>MPACCSWNDVLQYETNKVTRIQSTNYGTVKWVLHMIVFSYISFALVSDKLYQRKEPVISSVHTKVKGIAEVTENVTEGGVTKLGHSIFDTADYTFPLQGNSFFVMTNYVKSEGQVQTLCPEYPRRGAQCSSDRRCKKGWMDPQSKGIQTGRCVPYDKTRKTCEVSAWCPTEEEKEAPRPALLRSAENFTVLIKNNIHFPGHNYTTRNILPTMNGSCTFHKTWDPQCSIFRLGDIFQEAGENFTEVAVQGGIMGIEIYWDCNLDSWSHHCRPRYSFRRLDDKNTDESFVPGYNFRYAKYYKENNVEKRTLIKAFGIRFDILVFGTGGKFDIIQLVVYIGSTLSYFGLATVCIDLLINTYSSAFCRSGVYPYCKCCEPCTVNEYYYRKKCESIMEPKPTLKYVSFVDEPHIRMVDQQLLGKSLQVVKGQEVPRPQMDFSDLSRLSLSLHDSPLTPGQSEEIQLLHEEVAPKSGDSPSWCQCGNCLPSRLPEQRRALEELCCRRKPGRCITTSKLFHKLVLSRDTLQLLLLYQDPLLVLGEEATNSRLRHRAYRCYATWRFGSQDMADFAILPSCCRWRIRKEFPKTEGQYSGFKYPY[3x]

The P2X7 receptor is an ATP-gated ion channel that activates inflammatory pathways involved in diseases such as cancer, atherosclerosis, and neurodegeneration. When present in high concentrations, such as in pathological inflammatory states, extracellular ATP acts as a danger signal to cells by binding to and activating the P2X7 receptor (P2X7R). This spatiotemporal signaling stimulates the innate immune system by triggering assembly of the NLRP3 inflammasome and subsequent cytokine release, as well as activation of various less understood signaling cascades, ultimately resulting in apoptosis. P2X7R antagonists bind to either classical or extended allosteric ligand-binding sites that exist within the extracellular domain at the interface of two protomers.

To characterize the molecular differences between key mammalian P2X7R orthologs, we obtained cryo-EM structures of the full-length wild-type mP2X7 (2.5 Å) and hP2X7 (2.5 Å) receptors in the apo closed state conformation. Conserved features include their trimeric architecture, the 310-helices forming a closed gate, a partially hydrated sodium ion present in the closed pore, palmitoylation of residues in the C-cys anchor, and zinc and guanosine nucleotide-binding sites in the cytoplasmic ballast. There are also hydrogen bonds between the hemisuccinate group of the outer CHS molecule and the side chains of N261, H268, and K49 (distances of 2.8 Å, 3.4 Å, and 3.3 Å, respectively). Although all three ortholog reconstructions are of similar resolution (~2.5 Å), there are no densities in either the rP2X7R or the mP2X7R reconstructions to support modeling of CHS molecules, suggesting that these bound CHS molecules are specific to the hP2X7R. However, the identity of three residues within the classical allosteric pocket are different between human, mouse, and rat orthologs as seen in sequence alignments and visualized in their respective structures. Second, F108 in hP2X7Rs correlates to Y108 in both mP2X7Rs and rP2X7Rs. Finally, V312 in hP2X7Rs correlates to A312 in both mP2X7Rs and rP2X7Rs. The larger valine side chain in the human ortholog occupies more space within the classical allosteric pocket than the alanine in rat or mouse P2X7Rs. Residue I214 in hP2X7Rs and rP2X7Rs corresponds to a glycine in mP2X7Rs, introducing flexibility in the mouse ortholog that could explain some pharmacological differences. The larger side chain of V312 in the hP2X7R (A312 in the rP2X7R and the mP2X7R) forces an alternative rotameric conformation of Y295 compared to its conformation in the mP2X7R or the rP2X7R.> DKKLFLKRDNLLIADIELGCGNFGSVRQGV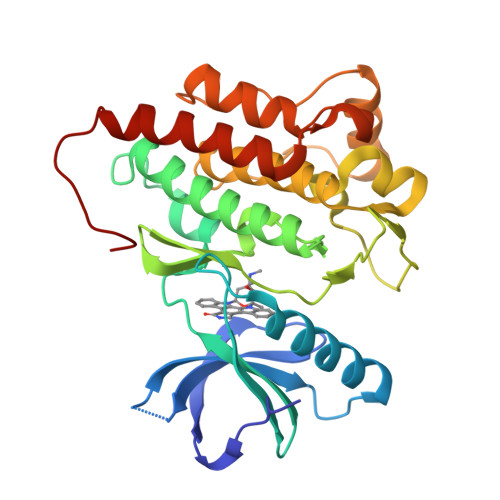YRMRKKQIDVAIKVLKQGTEKADTEEMMREAQIMHQLDNPYIVRLIGVCQAEALMLVMEMAGGGPLHKFLVGKREEIPVSNVAELLHQVSMGMKYLEEKNFVHRDLAARNVLLVNRHYAKISDFGLSKALGADDSYYTARSAGKWPLKWYAPECINFRKFSSRSDVWSYGVTMWEALSYGQKPYKKMKGPEVMAFIEQGKRMECPPECPPELYALMSDCWIYKWEDRPDFLTVEQRMRACYYSLASKVEGHHHHHHH>[5x]MPKITRDQVKVPADVLADARETYIDNYMKATQGTGRLMLFACDQKVEHLNGDFYGEGIDISDSDPEHLFKIADQGVCGVMAGQRGLIARYAADYPNVNYLVKMNSKTNLVKTAQDDPYSPQLH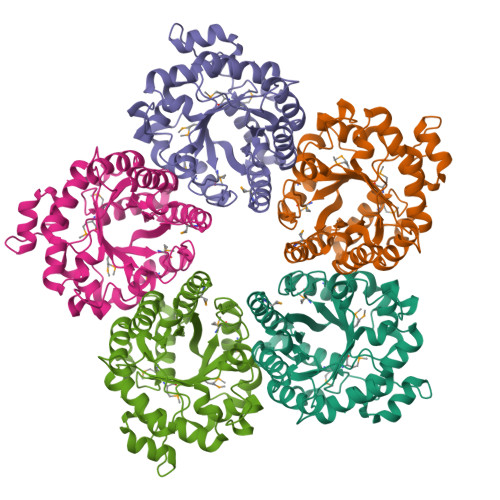DIEAVLAMRDNGVNVVGLGYTLYLGSEYEATMLAEAGQLVAQAHEEGLIVVLWIYPRGKAVGKDEKAPTTIAGAAGVALCLGADFVKVNPPVATEDKTSAENLAVASAAAGRTGLVCAGGSTVEAKVFLQQLHDQIYIGGASGNATGRNIHQRSLDEAVRLTKAISAITLADYDVDRALAVFNGEEDFALHHHHHH> GPMGNGMNKILPGLYIGNFKD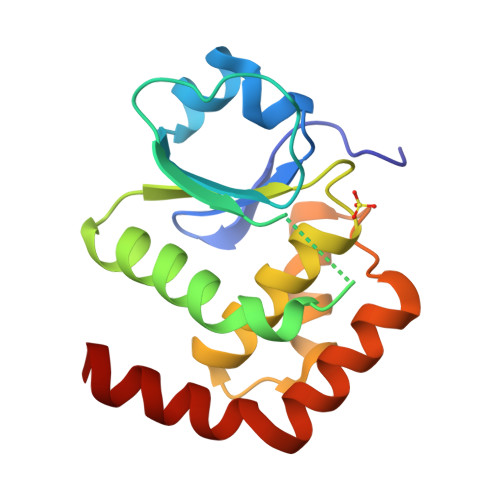ARDAEQLSKNKVTHILSVHDSARPMLEGVKYLCIPAADSPSQNLTRHFKESIKFIHECRLRGESCLVHCLAGVSRSVTLVIAYIMTVTDFGWEDALHTVRAGRSCANPDVGFQRQLQEFEKHEVHQYRQWLKEEYG> MVPISPIETVPVKLKPGMDGPKVKQWPLTEEKIKALVEICTEMEKEGKISKIGPENPYNTPVFAIKKKDSTKWRKLVDFRELNKRTQDFWEVQLGIPHPAGLKKKKSVTVLDVGDAYFSVPLDEDFRKYTAFTIPSINNETPGIRYQYNVLPQGWKGSPAIFQSSMTKILEPFAAQNPDIVIYQYMDDLYVGSDLEIGQHRTKIEELRQHLLRWGLTTPDKKHQKEPPFLWMGYELHPDKWTVQPIVLPEKDSWTVNDIQKLVGKLNWASQIYPGIKVRQLSKLLRGTKALTEVIPLTEEAELELAENREILKEPVHGVYYDPSKDLIAEIQKQGQGQWTYQIYQEPFKNLKTGKYARMRGAHTNDVKQLTEAVQKITTESIVIWGKTPKFKLPIQKETWETWWTEYWQATWIPEWEFVNTPPLVKLWYQLEKEPIVGAETFYVDGAANRETKLGKAGYVTNKGRQKVVPLTNTTNQKTELQAIYLALQDSGLEVNIVTDSQYALGIIQAQPDKSESELVNQIIE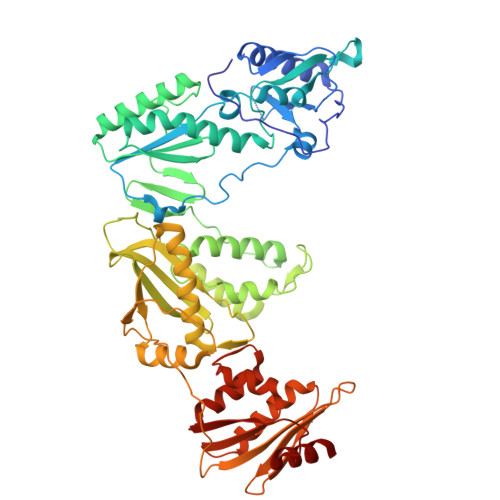QLIKKEKVYLAWVPAHKGIGGNEQVDKLVSAG>NPCLTGPRTCKDLLDRGHFLSGWHTIYLPDCRPLTVLCDMDTDGGGWTVFQRRVDGSVDFYRDWATYKQGFGSRLGEFWLGNDNIHALTAQGTSELRTDLVDFEDNYQFAKYRSFKVADEAEKYNLVLGAFVEGSAGDSLTFHNNQSFSTKDQDNDLNTGNCAVMFQGAWW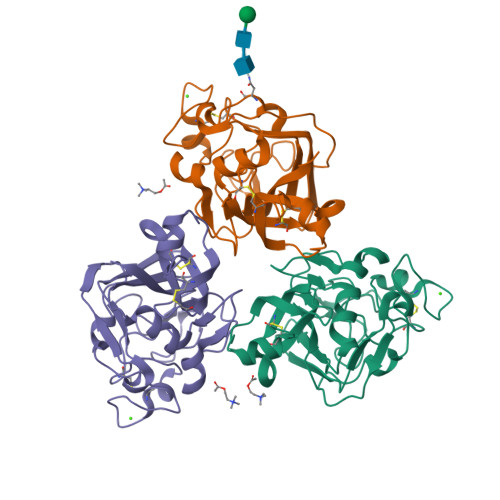YKNCHTSNLNGRYLRGTHGSFANGINWKSGKGYNYSYKVSEMKVRPA[6x]>MHHHHHHITSLYKKAGSEFALDSSKLEAIYATSEADRDYKENAVDGDENTIWHSAYQAADKLPVSITIKLDKAYDLNQIDYLPRQNSRNGHVTEYKIETSLDNENWTEVRTGNLEVNEAGNALANRGYNPIRFNTINAQYLRFTALKTLGDTNNKYASAAELVFYGK[2x]

As part of the secreted C. perfringens CAZyme arsenal, the bacterium possesses an open reading frame coding for a 220-kDa family 31 glycoside hydrolase (locus tag CPF_1301 in strain ATCC 13124) with predicted α-glucosidase activity, which will be hereafter referred to as CpGH31. In addition to the N-terminal glycoside hydrolase family 31 catalytic module, CpGH31 comprises two fibronectin-type III modules, three CBM32s, a putative cohesin module, and a bacterial immunoglobulin-like 2 module. Though the putative CBMs, referred to as CBM32-1, CBM32-2, CBM32-3, themselves are not closely related at the amino acid sequence level, a primary structure comparison indicates that they all belong to CBM family 32, an observation that is supported by their overall similar structures as determined by X-ray crystallography. Each CpGH31 CBM32 structure comprised the β-sandwich topology characteristic of this CBM family with a short α-helix and a calcium ion capping one side of each module.

The molecular determinants of galacto-specific sugar recognition displayed by CpGH31 CBM32-3 were revealed by the X-ray crystal structures of this protein module in its apo-, galactose-bound, and GalNAc-bound states, which were determined to 1.58 Å, 1.48 Å and 2.50 Å resolution, respectively. The galactose and GalNAc residues were well-ordered in the crystal structures of the CBM32-3:Gal and CBM32-3:GalNAc complexes, respectively, and provided clear electron density, allowing for monosaccharide modeling into each structure. The galactose and GalNAc coordinating amino acid residues of CBM32-3 were conserved, and included Tyr1674, His1671, Arg1702, Asn1707 and Tyr1774. The b-face of both sugars formed CH-π interactions with Tyr1674, while a secondary aromatic residue, Tyr1774, whose side chain is perpendicular to that of Tyr1674, mediated additional hydrophobic interactions with the C6 group of each sugar. Galactose and GalNAc binding was further stabilized through a series of polar contacts formed between the side chains of His1671, Arg1702 and Asn1707 and the C2-C3-C4-C5 edge of each sugar. Specifically, hydrogen bonds were observed between Asn1707 and the O4 hydroxyl and endocyclic oxygen, His1671 and the O4 hydroxyl, and Arg1702 and the O3 and O4 hydroxyl and 2-acetamido groups. The C6 of galactose is well-positioned to interact with the hydrophobic region formed by the adjacent side chains of Tyr1774 and Tyr1674, leaving the C1 of the sugar directed toward the solvent, which would allow for the binding of the β1-4-coordinated dissacharide LacNAc at this position. Although this residue is not conserved in CpGH31 CBM32-3, the side chain of Asp1769 is similarly positioned in an adjacent loop and could form hydrogen bond contact LacNAc. Alignment of the three CBM32-3 structures revealed minimal sugar—induced structural changes (backbone r.m.s.d < 0.22 Å) and only subtle differences in B-factors associated with the variable loops were also observed.> HAFRYSLNYPNIGHCIIINNKNFDRRTGMNPRNGTDVDAGNVMNVFRKLGYIVKVYNDQTVAQIMQVLTTVAHDDHSRCASLVCVLLSHGDEGVF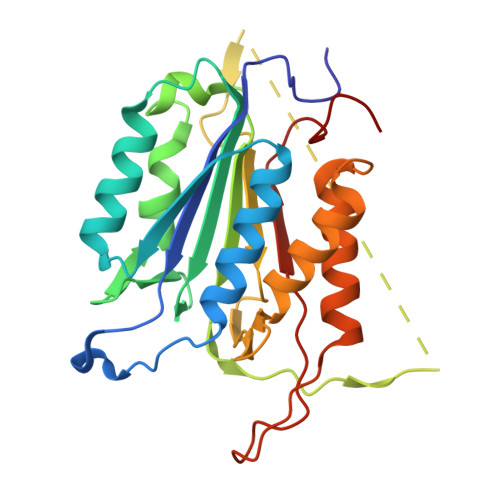FGTDTSVDLKSLTSLFRGDRCPSLVGKPKLFFIQACRGTELDPGVETDHTDHPDIPDGRERIPVEADFLYAYSTVPGYYSWRNTMTGSWFIQSLCEMMTKYGSELELLQIMTRVNHKVALDFESTSNMPGFDAKKQIPCIVSMLTKEMYFTPSE>GPPILKELENLSPEEAAHQKAVVETLLQEDPWRVAKMVKSYLQQHNIPQREVVDTTGLNQSHLSQHLNKGTPMKTQKRAALYT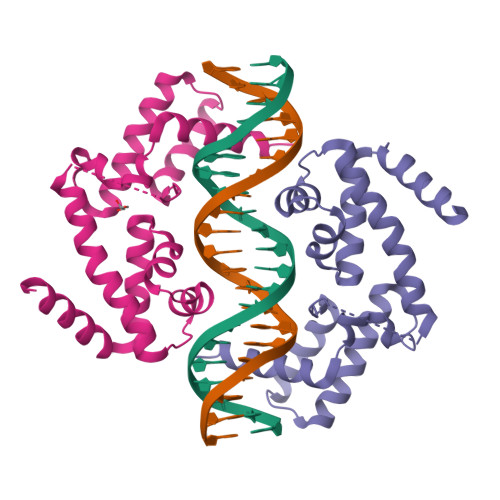WYVRKQREVAQQFTHAGQGGLIEEPTGDELPTKKGRRNRFKWGPASQQILFQAYERQKNPSKEERETLVEECNRAECIQRGVSPSQAQGLGSNLVTEVRVYNWFANRRKEEAFRH[2x]> TIGSEFKPHISALNAPSLAQRYKDYFYIGAAVEPYQTTKEKDAKMLQRHFNMIVAENAMKPAALEPTEGNFQWADADRIVQFAKENGMELRFHTLVWHNQTPDWFFLDREGKPMVEETDPQKREENRELLLQRLENHIRAVVLRYKDDIKNWDVVNEVVEPNDPGGMRNSPWYQITGTEYIEVAFRAAREAGGEDIKLYMNDYNTEQEPKREYIYRLIKKLLEKGVPIDGVGHQAHVTIDRPPVDEIKKTIQRFADLGLDNQITELDVSLYGWPPRPAYPTYDAIPEERFQAQADRYRQLFELFEELKDHISAVTFWGIADNHTWLDDRAREYNDGVGKDAPFVFDPNYRVKPAYWAIINHK

GH10 enzymes hydrolyze the β-1,4 glycosidic bonds linking the xyloside units that comprise the backbone of the polysaccharide xylan, which is second only to cellulose in abundance in the plant cell wall; xylanases are, therefore, essential for biomass degradation. The design method is inspired by the evolution of new enzymes in nature through recombination, insertion, deletion, and mutation. It starts by computationally segmenting all structures belonging to a modular enzyme family along structurally conserved sites and assembling the resulting modular fragments to generate a huge combinatorial diversity of backbones. Instead of using the natural sequences of the fragments, as in natural evolution or laboratory genetic recombination, we next design the sequence of the entire protein (>300 amino acids) to maximize compatibility between the fragments and stabilize the active-site geometry.

We then selected the eight most active designs and two natural GH10 enzymes for quantitative kinetic analysis with the chromogenic substrate 4-nitrophenyl β-xylobioside (O-PNPX2). The active designs spanned five orders of magnitude in catalytic efficiency. For instance, the most active GH10 design xyl3.1 and the least active one xyl8.3 exhibited OPNPX2 hydrolysis efficiencies of 9417 and 0.61 M-1 s-1, respectively. To understand what were the underlying structural reasons for this vast difference in efficiency, we determined their crystallographic structures. In both structures, the two catalytic Glu residues were positioned as in the design conception (<0.5 Å all-atom root-mean-square deviation (rmsd)). By contrast, the low-activity design xyl8.3 showed conformational changes in the residues that form the active-site hydrogen-bond network (2 Å all-atom rmsd). Furthermore, missing electron density in β-α loops 7 and 8 suggested that at least parts of the active-site pocket were mobile, although design accuracy was high throughout the segments of the design model and experimental structure that could be aligned (0.9 Å backbone rmsd). We, therefore, concluded that accurate positioning of the two catalytic Glu residues was crucial to obtain any level of activity, and that high levels of activity depended on atomic precision and preorganization in a large network of polar residues that surround the catalytic residues.3-oxo-N-[(3S)-2-oxooxolan-3-yl]tetradecanamide 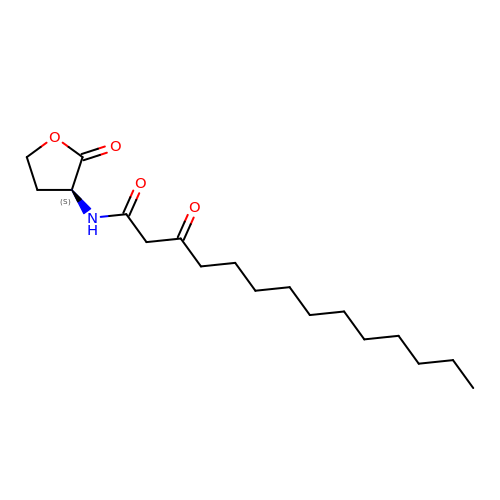| C18 H31 N O4 | YQFJJDSGBAAUPW-INIZCTEOSA-N>GPGSQYFRESILNDIRKARNLYTGKELAAELARIRQRVDNIEVLTADIVINLLLSYRDIQDYDSIVKLVETLEKLPTFDLASHHHVKFHYAFALNRRNLPGDRAKALDIMIPMVQSEGQVASDMYCLVGRIYKDMFLDSNFTDTESRDHGASWFKKAFESEPTLQSGINYAVLLLAAGHQFESSFELRKVGVKLSSLLGKKGNLEKLQSYWEVGFFLGA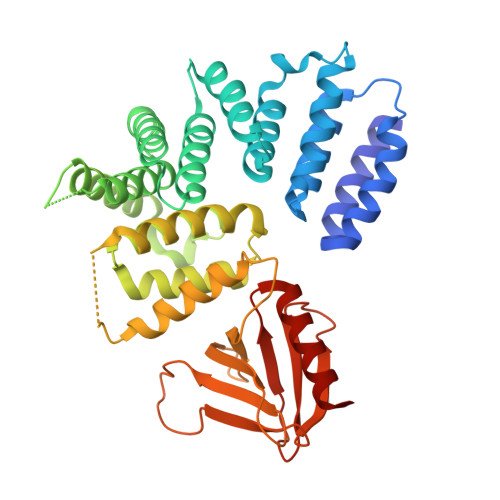SVLANDHMRVIQASEKLFKLKTPAWYLKSIVETILIYKHFVKLTTEQPVAKQELVDFWMDFLVEATKTDVTVVRFPVLILEPTKIYQPSYLSINNEVEEKTISIWHVLPDDKKGIHEWNFSASSVRGVSISKFEERCCFLYVLHNSDDFQIYFCTELHCKKFFEMVNTITEEKG[2x]> GPGSQELCLHERQRYRGLFAALAQTPSEEIAIVRSLSVPLVKTTPVSLPFCLDQTVADNCLTLSGMGYYLGIGGCCPACNAGDGRFAATSREALILAFVQQINTIFEHRAFLASLVVLADRHNAPLQDLLAGILGQPELFFVHTILRGGGACDPRLLFYPDPTYGGHMLYVIFPGTSAHLHYRLIDRMLTACPGYRFVAHVWQSTFVLVVRR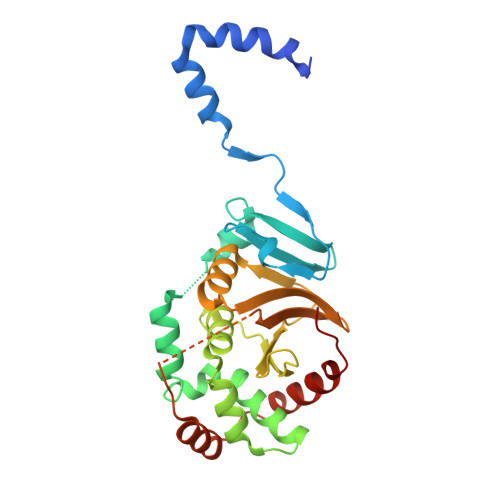NAEKPTDAEIPTVSAADIYCKMRDISFDGGLMLEYQRLYATFDEFPPP>[2x]MVLGKPQTDPTLEWFLSHCHIHKYPSKSTLIHQGEKAETLYYIVKGSVAVLIKDEEGKEMILSYLNQGDFIGELGLFEEGQERSAWVRAKTACEVAEISYKKFRQLIQVNP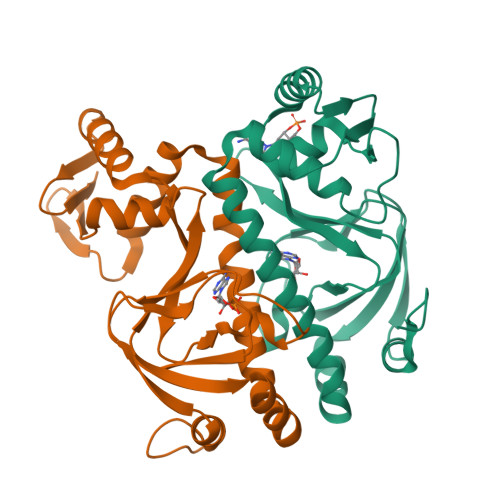DILMRLSAQMARRLQVLAEKVGNLAFLDVTGRIAQTLLNLAKQPDAMTHPDGMQIKITRQEIGQIVGCSRETVGRILKMLEDQNLISAHGKTIVVYGTR> SAKDLDAVDAILE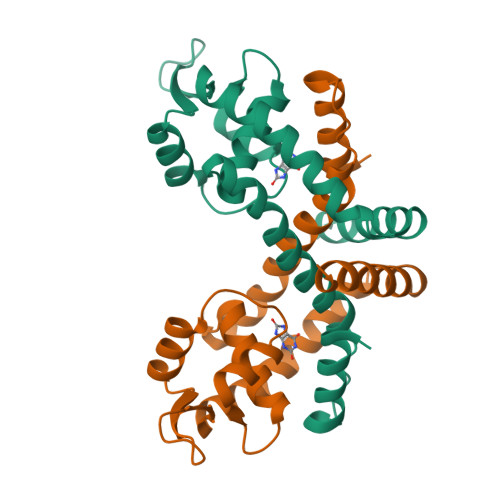QWRRERPDLDASPMGPIGRLRRCAVLMDQRLESCFSRFDLSSWEFDMLATLRRAGAPHCLSPTELFSTLMVTSGTMTHRLKRLETRGFIERVQNELDARSTLVQLTSSGLELINRAVEAHIENERQVLSVLPAEVLAALDTNLAALLRGLESHNKGN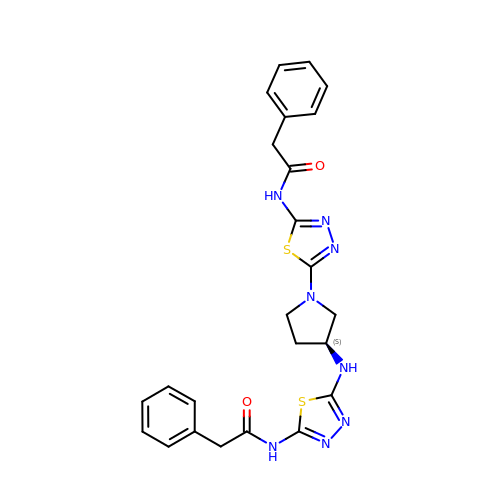2-phenyl-~{N}-[5-[[(3~{S})-1-[5-(2-phenylethanoylamino)-1,3,4-thiadiazol-2-yl]pyrrolidin-3-yl]amino]-1,3,4-thiadiazol-2-yl]ethanamide | C24 H24 N8 O2 S2 | XKAUHJUBYCZSGD-SFHVURJKSA-N>GT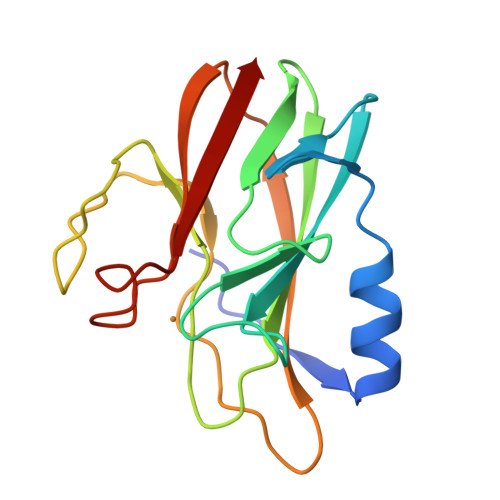LDTTWKEATLPQVKAMLEKDTGKVSGDTVTYSGKTVHVVAAAVLPGFPFPSFEVHDKKNPTLEIPAGATVDVTFINTNKGFGHSFDITKKGPPYAVMPVIDPIVAGTGFSPVPKDGKFGYTNFTWHPTAGTYYYVCQIPGHAATGQFGKIVVK[2x]> GSHVSIDQIDLIHDIEHVIQQFPTVRFTFNKNNGQLFLIGHVRNSIDKSELLYKVDALS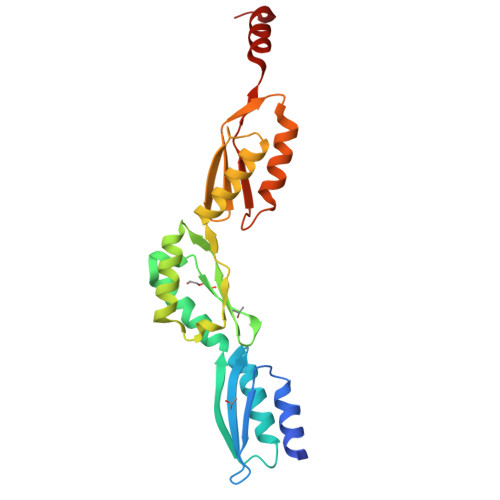FVKSVDDNVIDDEAVWQEMNILLSKNPEFKGISMQSPEPGIFVISGYLKTEEQAACLADYLNLHFNYLSLLDNKVIIESQVMKALAGHLVQSGFANVHVSFTNGEAVLTGYINNKDADKFRTVVQELQDIAGIRAVKNFVVLLPAEEGVIDLNMRYPG>MQNETINLKQHLAAIKEYWQPEIINRHGFQFHLVKLLGDYGWHTHGYSDKVLFAVEGDMAVDF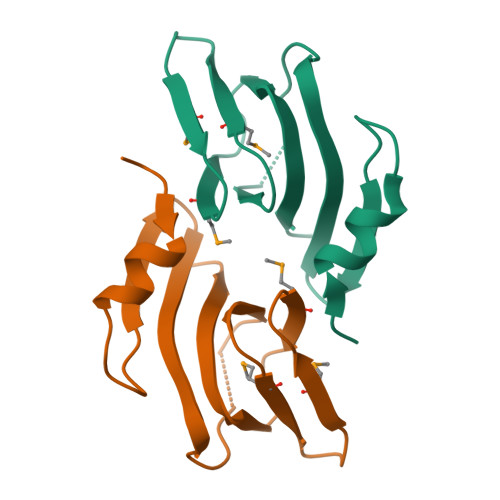ADGGSMTIREGEMAVVPKSVSHRPRSENGCSLVLIELSDPSEAV[10x]>[5x]QDMVSPPPPIADEPLTVNTGIYLIECYSLDDKAETFKVNAFLSLSWKDRRLAFDPVRSGVRVKTYEPEAIWIPEIRFVNV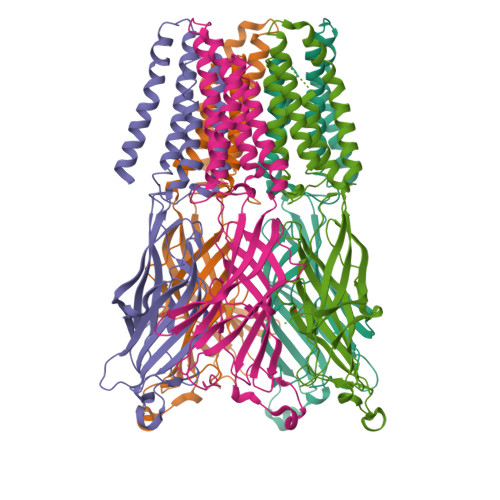ENARDADVVDISVSPDGTVQYLERFSARVLSPLDFRRFPMDSQTLHIYLIVRSVDTRNIVLAVDLEKVGKNDDVFLTGWDIESFTAVVKPANFALEDRLESKLDYQLRISRQMGYYLIQMYIPSLLIVILSWISFWINMDAAPARVGLGITTVLTMTTQSSGSRASLPKVSYVKAIDIWMAVCLLFVFSALLEYAAVNFVSRQSQPQRAKKIDKISRIGFPMAFLIFNMFYWIIYFGFGGHHHHHHHHHH> MEKFVLSLDEGTTSARAIIFDRESNIHGIGQYEFPQHYPRPGWVEHNPEEIWDAQLRAIK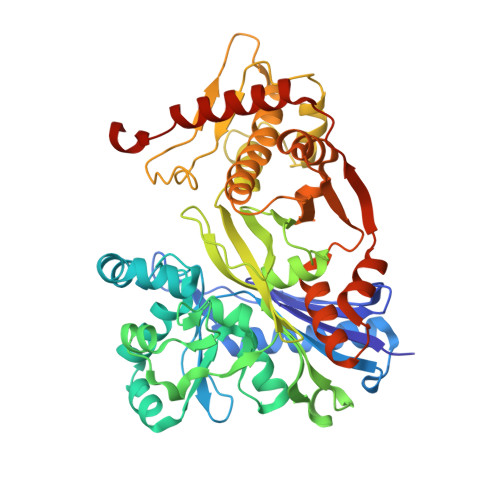DAIQSARIEPNQIAAIGVTNQRETTLVWDKDGKPLYNAIVWQCRRTAEMVEEIKREYGTMIKEKTGLVPDAYFSASKLKWLLDNVPGLREKAEKGEVMFGTVDTFLIYRLTGEHVTDYSNASRTMLFNIKKLDWDDELLELFDIPESVLPEVRESSEVYGYTKKELLGAEIPVSGDAGDQQAALFGQAAFEAGMVKATYGTGSFILVNTDEMVLYSDNLLTTIAWGLNGRVSYALEGSIFVTGAAVQWLRDGIKIIKHASETEELATKLESNEGVYFVPAFVGLGAPYWDQFARGIIIGITRGTGREHLARATLEAIAYLTRDVVDEMEKLVQIKELRVDGGATANDFLMQFQADILNRKVIRPVVKETTALGAAYLAGLAVDYWADTREIAELWKAERIFEPKMDEKTRERLYKGWKEAVKRAMGWAKVVDSAKSN> MHHHHHHHHHHSGDEVDAGSGHMGTQKVTPALIFAITVATIGSFQFGYNTGVINAPEKIIKEFITKTLTDKGNAPPSEVLLTSLWSLSVAIFSVGGMIGSFSVGLFVNRFGRRNSMLIVNLLAVTGGCFMGLCKVAKSVEMLILGRLVIGLFCGLCTGFVPMYIGEISPTALRGAFGTLNQLGIVVGILVAQIFGLEFILGSEELWPLLLGFTILPAILQSAALPFCPESPRFLLINRKEEENAKQILQRLWGTQDVSQDIQEMKDESARMSQEKQVTVLELFRVSSYRQPIIISIVLQLSQQLSGINAVFYYSTGIFKDAGVQEPIYATIGAGVVNTIFTVVSLFLVERAGRRTLHMIGLGGMAFCSTLMTVSLLLKDNYNGMSFVCIGAILVFV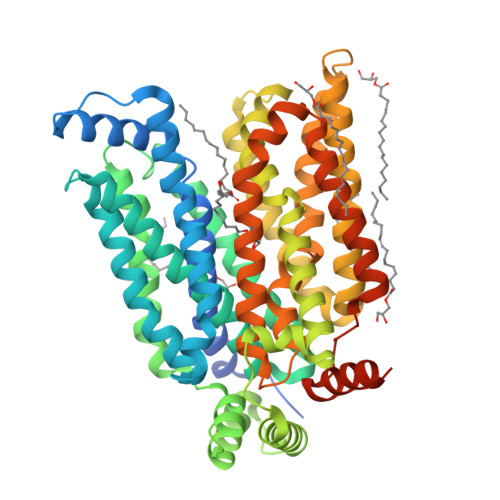AFFEIGPGPIPWFIVAELFSQGPRPAAMAVAGCSNWTSNFLVGLLFPSAAHYLGAYVFIIFTGFLITFLAFTFFKVPETRGRTFEDITRAFEGQAHGADRSGKDGVMEMNSIEPAKETTTNV> AAAAKGIAI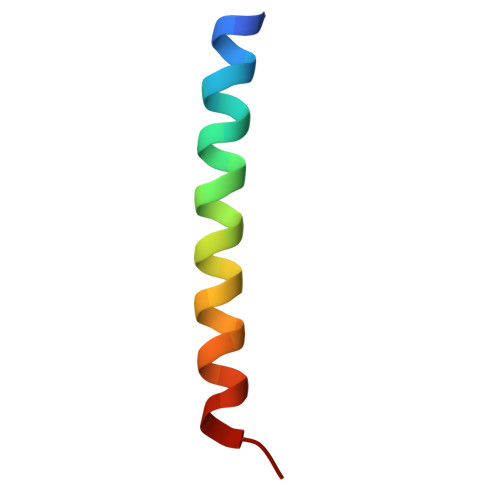ALLVILVICSLIVTSVILLTPA~{N}-(1,4-dimethyl-2-oxidanylidene-quinolin-7-yl)methanesulfonamide 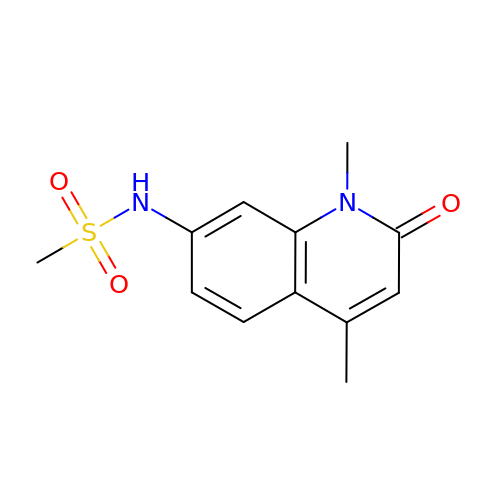| C12 H14 N2 O3 S | LJTKZAIXTKZSBU-UHFFFAOYSA-N>[2x]GMTTNTIMEQEARTAPQKIAEQLLANDAITESLGSVLREFKPKFVMIVGRGSSDHAGVFAKYLFEIEASIPTFAAAPSVASVYGKTLK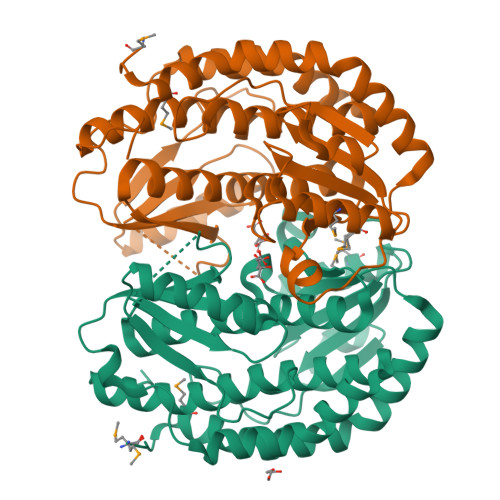LAGGLVIVISQSGRSPDILAQARMAKNAGAFCVALVNDETAPIKDIVDVVIPLRAGEEKAVAATKSYLATLSALLQVAAKWTQNESLVEAVNSLPQALQAAVDAEPQLRAGSLTDVKNLVVLGRGFGYAVSKEIALKLKEVCAIHAEAFSSAEFLHGPVTLVEKKLSILDVCIRDESYGSHVEQIANVKQRGANLIHLHQTSADIHPRIAPLALLQRFYIDVAAVAIALGINPDKPAGLKKVTQTL>HHAALRQPQVAELLAEARRAFREEFGAEPELAVSAPGRVNLIGEHTDYNQGLVLPMALELMTVLVGSPRKDGLVSLLTTSEGADEPQRLQFPLPTAQRSLEPGTPRWANYVKGVIQYYPAAPLPGFSAVVVSSVPLGGGLSSSASLEVATYTFLQQLCPDSGTIAARAQVCQQAEHSFAGMPCGIMDQFISLMGQKGHALLIDCRSLETSLVPLSDPKLAVLITNSNVRHSLASSEYPVRRRQCEEVARALGAASLREVQLEELEAARDLVSKEGFRRARHVVGEIRRTAQAAAALRRGDYRAFGRLMVESHRSLRDDYEVSCPELDQLVEAALAVPGV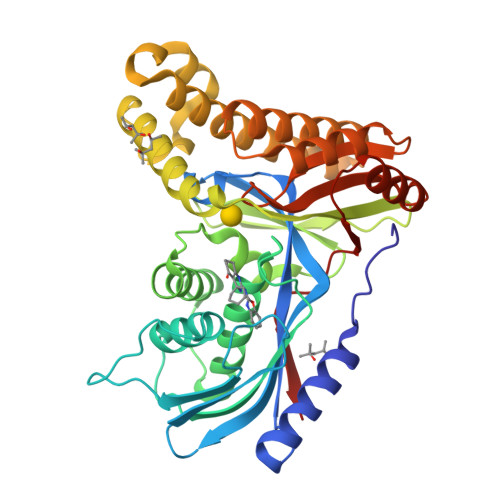YGSRMTGGGFGGCTVTLLEASAAPHAMRHIQEHYGGTATFYLSQAADGAKVLCL[2x]4-[(4,4-dimethylpiperidin-1-yl)methyl]-~{N}-[[(3~{R})-1-[6-(methylamino)pyrimidin-4-yl]-3-oxidanyl-piperidin-3-yl]methyl]-2-oxidanyl-benzamide 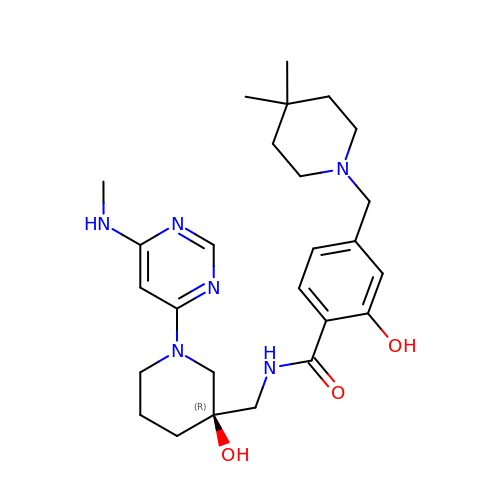| C26 H38 N6 O3 | BEGALFNTKBNFJE-AREMUKBSSA-N> GLPTELKPGTNQFLTTDDGTSPPILPGFEPTPLIHIPGEFTSLLDLCRIETILEVNNTTGTTGVNRLLIPVRAQNNVDQLC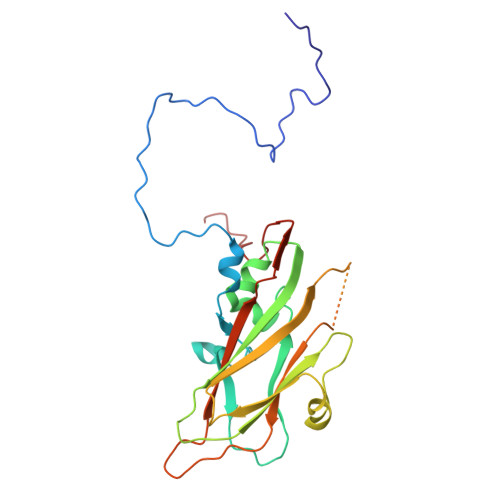ASFQVDPGRNGPWQSTMVGQICRYYTQWSGSLKVTFMFTGSFMATGKMLIAYTPPGSAQPTTREAAMLGTHIVWDFGLQSSVTLVIPWISNTHFRAVKTGGVYDYYATGIVTIWYQTNFVVPPDTPSEANIIALGAAQENFTLKLCKDTDEIRQTAEYQ> RGSHMLEMIIKPRVRGFICVTAHPTGCEANVKKQIDYVTTEGPIANGPKRVLVIGASTGYGLAARITAAFGCGAD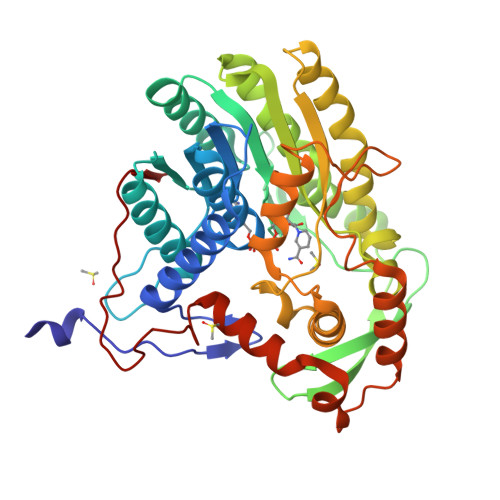TLGVFFERPGEEGKPGTSGWYNSAAFHKFAAQKGLYAKSINGDAFSDEIKQLTIDAIKQDLGQVDQVIYSLASPRRTHPKTGEVFNSALKPIGNAVNLRGLDTDKEVIKESVLQPATQSEIDSTVAVMGGEDWQMWIDALLDAGVLAEGAQTTAFTYLGEKITHDIYWNGSIGAAKKDLDQKVLAIRESLAAHGGGDARVSVLKAVVCQASSAIPMMPLYLSLLFKVMKEKGTHEGCIEQVYSLYKDSLCGDSPHMDQEGRLRADYKELDPEVQNQVQQLWDQVTNDNIYQLTDFVGYKSEFLNLFGFGIDGVDYDADVNPDVKIPNLIQG> GSTSARNHTEDNSTEYYDYEEARCACPARHLNNTNGTVLKPLGCHYFCNGTLCTAPDGYPCYNLTAQQVRTLTTYPNTSCAVGVCMKGTCVKNG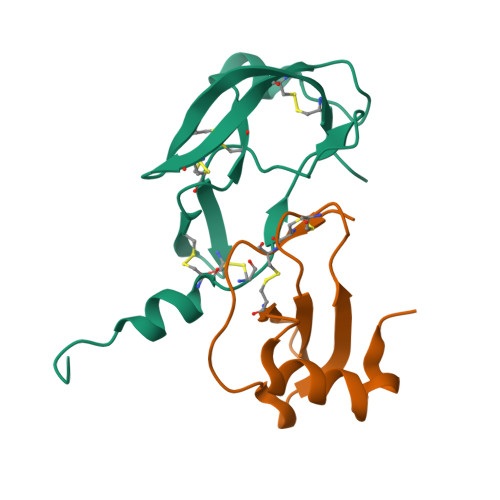TMEQCFKTP;> ARGTNVGRECCLEYFKGAIPLRKLKTWYQTSEDCSRDAIVFVTVQGRAICSDPNNKRVKNAVKYLQSLERS> MAR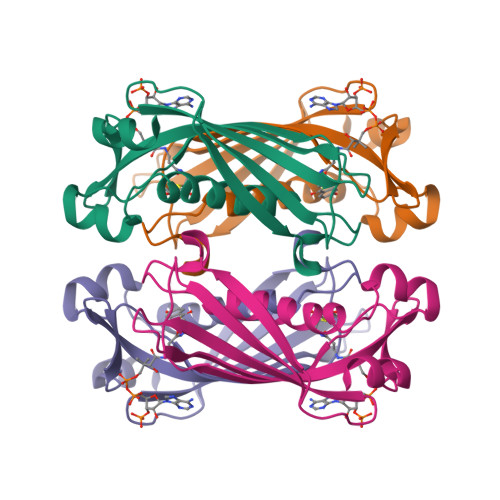SITMQQRIEFGDCNPAGIVWYPNYHRWLDAASRNYFIKCGLPPWRQTVVERGIVGTPIVSCNASFVCTASYDDVLTIETCIKEWRRKSFVQRHSVSRTTPGGDVQLVMRADEIRVFAMNDGERLRAIEVPADYIELCS> MATGTRYAGKVVVVTGGGRGIGAGIVRAFVNSGARVVICDKDESGGRALEQELPGAVFILCDVTQEDDVKTLVSETIRRFGRLDCVVNNAGHHPPPQRPEETSAQGFRQLLELNLLGTYTLTKLALPYLRKSQGNVINISSLVGAIGQAQAVPYVATAGAVTAMTKALALDESPYGVRVNCISPGNIWTPLWEELAALMPDPRASIREGMLAQPLGRMGQPAEVGAAAVFLASEANFCTGIELLVTGGAELGYGCKASRSTPVDAPD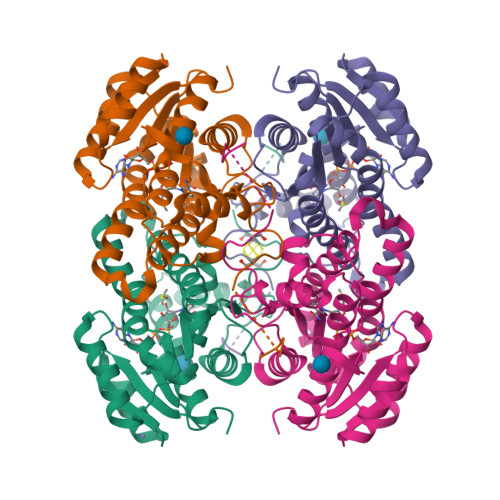IPS> MIKNEIKILSDIEHIKKRSGMYIGSSANETHERFMFGKWESVQYVPGLVKLIDEIIDNSVDEGIRTKFKFANKINVTIKNNQVTVEDNGRGIPQAMVKTPTGEEIPGPVAAWTIPKAGGNFGDDKERVTGGMNGVGSSLTNIFSVMFVGETGDGQNNIVVRCSNGMENKSWEDIPGKWKGTRVTFIPDFMSFETNELSQVYLDITLDRLQTLAVVYPDIQFTFNGKKVQGNFKKYARQYDEHAIVQEQENCSIAVGRSPDGFRQLTYVNNIHTKNGGHHIDCAMDDICEDLIPQIKRKFKIDVTKARVKECLTIVMFVRDMKNMRLIRQTKERLTSPFGEIRSHIQLDAKKISRDIL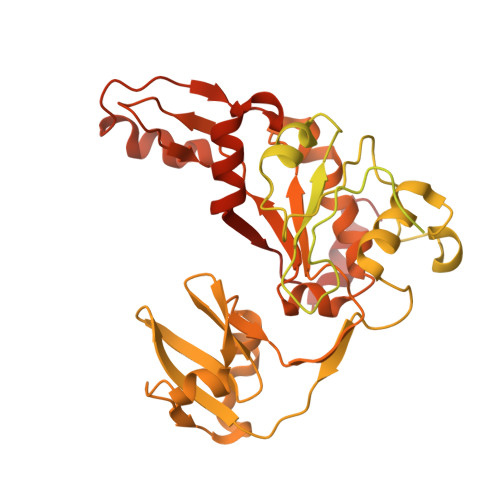NNEAILMPIIEAALARKLAAEKAAETKAAKKASKAKVHKHIKANLCGKDADTTLFLTEGDSAIGYLIDVRDKELHGGYPLRGKVLNSWGMSYADMLKNKELFDICAITGLVLGEKAFEEKEDGEWFTFELNGDTIIVNENDEVQINGKWITVGELRKNLMKFVKIDSSSVDMKKYKLQNNVRRSIKSSSMNYANVAIMTDADHDGLGSIYPSLLGFFSNWPELFEQGRIRFVKTPVIIAQVGKKQEWFYTVAEYESAKDALPKHSIRYIKGLGSLEKSEYREMIQNPVYDVVKLPENWKELFEMLMGDNADLRKEWMSQHHHHHH>[4x]MSILHMPLKIKDITIKNRIMMSPMCMYSASTDGMPNDWHIVHYATRAIGGVGLI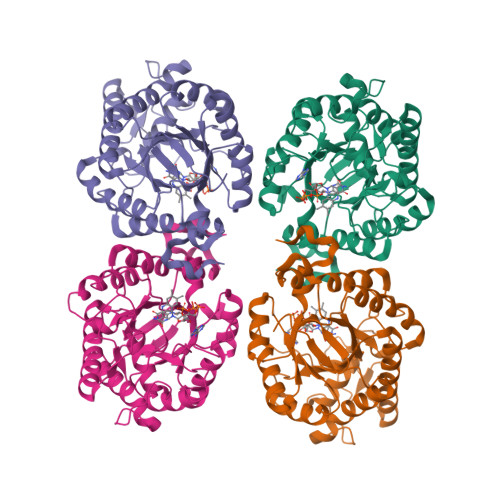MQEATAVESRGRITDHDLGIWNDEQVKELKKIVDICKANGAVMGIQLAHAGRKCNISYEDVVGPSPIKAGDRYKLPRELSVEEIKSIVKAFGEAAKRANLAGYDVVEIHAAHGYLIHEFLSPLSNKRKDEYGNSIENRARFLIEVIDEVRKNWPENKPIFVRVSADDYMEGGINIDMMVEYINMIKDKVDLIDVSSGGLLNVDINLYPGYQVKYAETIKKRCNIKTSAVGLITTQELAEEILSNERADLVALGRELLRNPYWVLHTYTSKEDWPKQYERAFKK> RSMFLPPPNYLFVRDVWKSNLYSEFAVIRQLVSQYNHVSISTEFVGTLARPIGTFRSKVDYHYQTMRANVDFLNPIQLGLSLSDANGNKPDNGPSTWQFNFEFDPKKEIMSTESLELLRKSGINFEKHENLGIDVFEFSQLLMDSGLMMDDSVTWITYHAAYDLGFLINILMNDSMPNNKEDFEWWVHQYMPNFYDLNLVYKIIQEFKNPQLQQSSQQQ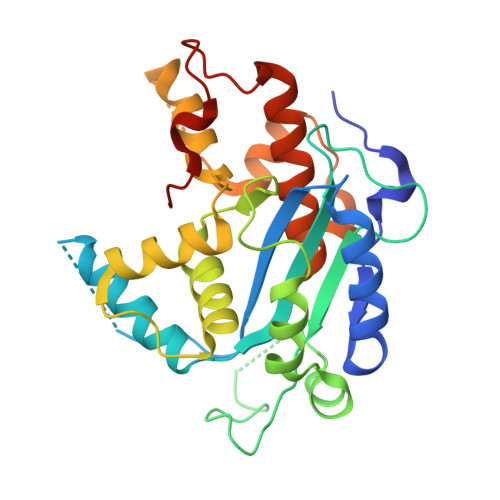QQQQYSLTTLADELGLPRFSIFTTTGGQSLLMLLSFCQLSKLSMHKFPNGTDFAKYQGVIYGIDGDQ>MAFNPAPKAVQENHHVDYVIRFNYGDIDTPEAIKKFEVLLLELSEVGLQTEVRQGDENSLFVFVRAASKKKLKRAVYQSRVRDWLYGVRNTEPEPASSAKPQSEAERLLVIYHLITVPKAEGGAGITPRHGEWKNVDAIFPLHDEETNRQCMREWSKKTFLSTEDLDRIRNTFGEHVGFYFAFLQSYFRFLMFPAAFGFSCWLLLGSFSIIYTVVNCLWCIVFIEYWKRQEEDLSCRWQTKGVSAVHEKRAEFKPEKEIRDESTGEVRGVFPATKRMYRQLLQVPFALLAAVALGAIIATCFAIEIFISEVYNGPLKGYLVFIPTILVSALIPTMSAVLLTVATKLNDYENYETQDAYKVALTQKIFVVNFITSYLPIILTAFVYVPFASRIVPYLDVFHLTVRPFVSKEHAIKARTEFSINPDRLRKQVIYFTVTAQIVGFALETIVPFVKQRVFREYKEYTKKQHAKAEPGNGAGEKKTVSLGDDEDEARFLTRVRNEAELEDYDVTDALRAMCIQFGYLALFSPVWPLVPVSFLINNWVELRSDFFKICVECKRPWPQRADTIGPWLDSLGFLSWVGS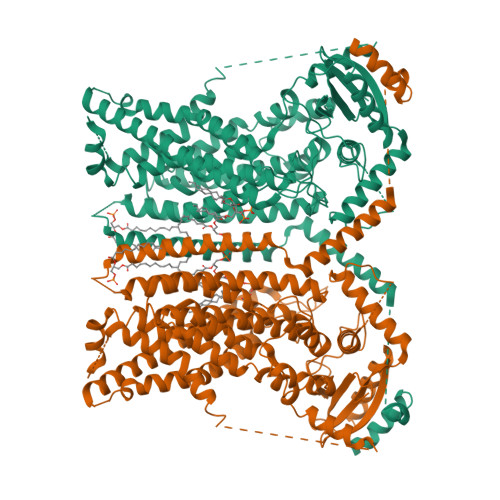ITSSALVYMFSNGHEGPNGEPTTIRCWALLLTIFFSEHLYLIVRYAVRSALAKLEPPNTRRERIERFMMRKRYLDTVLSAESDDDADEVKGVVSSIPPSEITRESLEQDARDWSKQGTDPTERFWMRQRGWKESAEVGLSLITKAKGDETKKQQ[2x]6-(4-methoxyphenyl)-N~4~,N~4~-bis[(pyridin-2-yl)methyl]pyrimidine-2,4-diamine | C23 H22 N6 O | 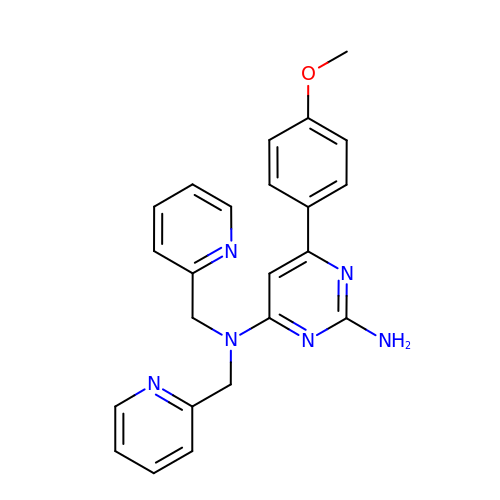FIGQTBBMNODYCB-UHFFFAOYSA-N> AERSLLTGEEGWRTYKATGPRLSLPRLVALLKGQGLEVGKVAEAEGGFYVDLRPEARPEVAGLRLEPARRVEGLLEIPSRTRRPARA

The ‘heat-resistant RNA-dependent ATPase’ Hera is a DEAD box protein from Thermus thermophilus. Hera consists of a helicase core, followed by a bipartite C-terminal extension that contains a dimerization domain (DD) and an RNA-binding domain (RBD). The RBD is responsible for binding of Hera to 23S rRNA fragments comprising hairpin 92 and for binding of RNaseP RNA. The Hera RBD forms a modified RNA recognition motif (RRM).

Crystals of Hera_RBD (residues 424-510) in complex with a tetranucleotide were obtained and the structure of the complex was determined to 2.3 Å resolution. The tetranucleotide must have been generated in situ by partial hydrolysis of the 19mer RNA. Based on clear electron density and hydrogen bonding distances, the sequence of the RNA could be assigned as 5′-GGGPyr-3′. The only GGGPyr element present in the 19mer RNA is a GGGC stretch, and GGGC was therefore modeled into the electron density. The RBD core adopts a similar structure in the RNA-free and RNA-bound form, in agreement with the secondary structure information from NMR. In the RBD/RNA complex structure, the C-terminal tail is visible up to aa 499, whereas the remainder appears to be disordered. Residues 492-499 pack closely to the RBD without engaging in contacts with the bound RNA. The 5′-guanine (Gua1) of the GGGPyr sequence is base-specifically bound by the N-terminal subdomain of Hera_RBD, a small addendum of 12 residues (A424-W435) unique to Hera. Further, the side-chain of K463 stacks against the side of Gua1, rationalizing the deleterious effect of the K463A mutation on RNA binding to the RBD (see previously). The second nucleotide, Gua2, binds through three hydrogen bonds of the Watson–Crick face to main-chain amide groups (V461, G462 and V464).> MAVTATILASSGGAKTTTAEADKFDYTVEQFADLQILRYKVPEFETLTLKQKELVYYLTQAALEGRDILFDQNGKYNLRIRRMLEAVYTNYKGDKSAPDFKNMEVYLKRVWFSNGIHHHYGMEKFVPGFSQDFLKQAVLGTDAQLLPLSEGQTAEQLSDELFPVMFDPAILAKRVNQADGEDLVLTSASNYYDGVTQQEAESFYGAMKDPKDETPVSYGLNSRLVKEDGKIQEKVWKVGGLYTQAIEKIVYWLKKAETVAENDAQKAVISKLIQFYETGSLKDFDEYAILWVKDLDSRIDFVNGFTESYGDPLGVKASWESLVNFKDLDATHRTEIISSNAQWFEDHSPVDKSFKKEKVKGVSAKVITAAILAGDLYPATAIGINLPNANWIRAHHGSKSVTIGNITDAYNKAAHGNGFNEEFVSNDEERQRIDQYGDLTGELHTDLHESLGHGSGKLLPGVDPDALKAYGSTIEEARADLFGLYYVADPKLVELKLVPDAEAYKAEYYTFLMNGLMTQLVRIEPGNNIEEAHMRNRQLIARWVFEKGAPDKVVEMVKKDGKTYVVVNDYEKVRQLFGELLAEIQRIKSTGDFEGARTLVENYAVKVDPALHAEVLARYKKLNLAPYKGFINPVYELVTDKDGNITDVTVSYNEDYVEQMLRYSKDYSPLPSVNNLEHHHHHH

DPP III (EC 3.4.14.4; earlier names: dipeptidyl arylamidase III, dipeptidyl aminopeptidase III) is a cytosolic zinc-metallopeptidase of the M49 family. This exopeptidase catalyses the hydrolysis of the penultimate peptide bond of its oligopeptide substrates with unsubstituted N-termini, thereby sequentially removing N-terminal dipeptides. Despite a low sequence identity (17–21%), the overall structure of BtDPP III is very similar to the previously reported crystal structures of human and yeast DPP III and consists of two domains separated by a wide cleft. The catalytic zinc ion is positioned in the lower part of the upper structural domain, coordinated by His448, His453, and Glu476.

Since we failed to obtain crystals from the purified wild-type protein, we assumed that the heterogeneity introduced by the oxidation of thiol groups had impeded crystallization. Thus, our results suggested that the observed charge heterogeneity in the purified BtDPP III was not caused by the oxidation of a single thiol group, but rather the outcome of oxidative modification of several thiol groups. Therefore, we prepared an additional variant with all five cysteine residues replaced by serine (Cys-null variant). As shown in Fig 1B (lane 11) this variant showed significantly improved homogeneity with one dominant protein form (position 11). Further crystallization screens were prepared using microseeding, and crystals of the Se-Met-labelled Cys-null protein were obtained in four new conditions: JCSG+ C10, E2, G11, and Midas G7. The best diffracting crystal was used for the complete data collection, and the crystal structure was solved using SAD at 1.9 Å resolution. The structure was solved at 2.4 Å resolution using molecular replacement, with the structure of the Cys-null variant as a search model. Both proteins crystallized in space group P3121, with one molecule in the asymmetric unit. By superimposing the wild-type on the Cys-null structures, we confirmed that the replacement of cysteine residues or the incorporation of Se-Met did not change the protein structure (backbone RMSD 0.15 Å). In the crystal structure of the Cys-null variant (open form), one Tris molecule, contained in the storage buffer, was bound to the zinc ion.The human pregnane X receptor (PXR, NR1I2) is a transcription factor belonging to the nuclear receptor (NR) family. Indeed, the PXRLBD contains a large and versatile ligand-binding pocket (LBP), which enables it to bind a range of molecules with different structures and chemical properties, thereby fulfilling its biological functions. PXR is traditionally regarded as a xenobiotic receptor, and as such it regulates the transcription of metabolizing enzymes and drug transporters, thereby facilitating the removal of xenobiotics from the body. To overcome this problem, we designed a new PXRLBD-Thb-SRC-1 fusion construct that combines the advantage of having good stability and solubility during purification with the possibility of crystallizing the PXRLBD with or without SRC-1 thanks to the introduction of a thrombin cleavage site between the PXRLBD and SRC-1 parts.

The difficulties encountered in obtaining a sufficient quantity of pure protein in a reproducible manner for use in crystallization trials prompted us to redesign the tethered construct. The novelty of this construct lies in the presence of a thrombin cleavage site in the junction region between the PXRLBD and SRC-1 parts, where the –GGSGG– sequence has been replaced by –LVPRGS–. In order to assess the usefulness of the new construct and to verify that the new linker does not affect the process of crystallization, we determined the structure of the PXRLBD in complex with the reference ligand SR12813 with and without the SRC-1 peptide. The crystals of the SR12813–PXRLBD-Thb-SRC-1 complex, which have the symmetry of space group P212121 with two molecules per asymmetric unit, were grown at 4°C in MPD, whereas those of the SR12813–PXRLBD complex have the symmetry of space group P43212, with one molecule per asymmetric unit, and were obtained at room temperature in 2-propanol. Only the SRC-1 peptide region interacting with the PXRLBD is well defined. Similarly, the region preceding H2′ (more or less including residues 176–209), which is absent in all of the PXRLBD and PXRLBD-SRC-1 structures listed in Table 1, is no more clearly defined in the new model. A closer examination of the LBP revealed that the SR12813 ligand maintains its original orientation and specifically interacts with the protein. These interactions involve the formation of hydrogen bonds to the side chains of residues Ser247 and His407.

>[2x]MKKGHHHHHHGSERTGTQPLGVQGLTEEQRMMIRELMDAQMKTFDTTFSHFKNFRLPGVLSSGCELPESLQAPSREEAAKWSQVRKDLCSLKVSLQLRGEDGSVWNYKPPADSGGKEIFSLLPHMADMSTYMFKGIISFAKVISYFRDLPIEDQISLLKGAAFELCQLRFNTVFNAETGTWECGRLSYCLEDTAGGFQQLLLEPMLKFHYMLKKLQLHEEEYVLMQAISLFSPDRPGVLQHRVVDQLQEQFAITLKSYIECNRPQPAHRFLFLKIMAMLTELRSINAQHTQRLLRIQDIHPFATPLMQELFGITGSLVPRGSSSHSSLTERHKILHRLLQEGSPS>[4x]GPLGSQPKTFTVRIVTMDAEMEFNCEM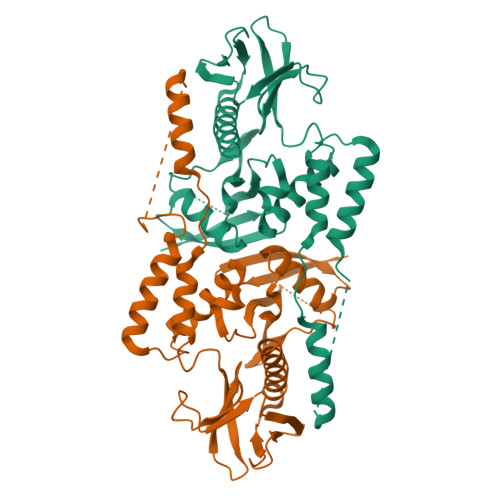KWKGKDLFDLVCRTLGLRETWFFGLQYTIKDTVAWLKMDKKVLDHDVSKEEPVTFHFLAKFYPENAEEELVQEITQHLFFLQVKKQILDEKIYCPPEASVLLASYAVQAKYGDYDPSVHKRGFLAQEELLPKRVINLYQMTPEMWEERITAWYAEHRGRARDEAEMEYLKIAQDLEMYGVNYFAIRNKKGTELLLGVDALGLHIYDPENRLTPKISFPWNEIRNISYSDKEFTIKPLDKKIDVFKFNSSKLRVNKLILQLCIGNHDLFMRRRK>GDWAPADVQAAL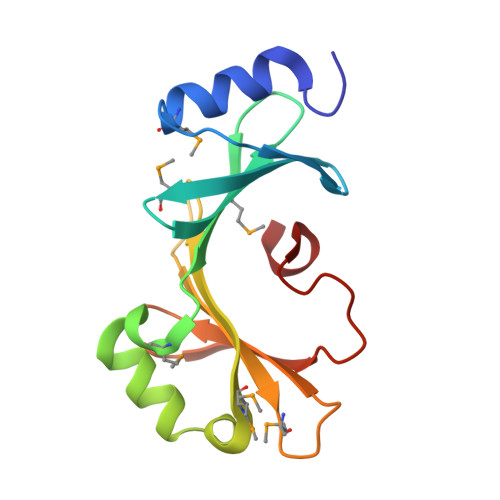KKMYPTADGVAWSHDESYYVADFLMNGFDTKVWFDGQAQWVMQQTDWETMDEVPPAVYNAFAASEYSGGMVQNVTWVQFPKWQSIVAVEVGMANLQTKYQILFTPTGEIIRARNVTYTYNPLGAATFL[2x]> MYNLHREKIFMSYNQNKQYLEDNPEIQEKIELYGLNLLNEVISDNEEEIRADYNEANFLHPFWMNYPPLDRGKMPKGDQIPWIEVGEKAVGSKLTRLVSQREDITVREIGLPTGPDERYLLTSPTIYSLTNGFTDSIMMFVDIKS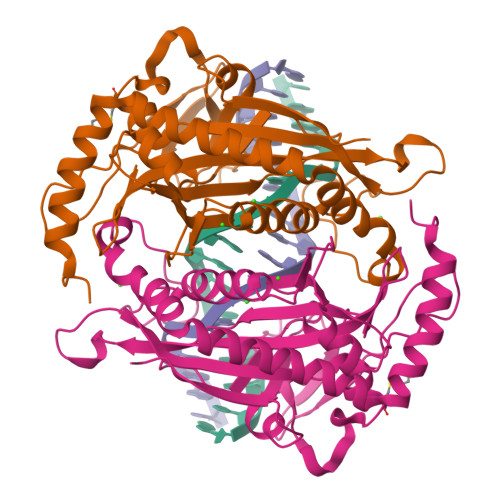VGPRDSDYDLVLSPNQVSGNGDWAQLEGGIQNNQQTIQGPRSSQIFLPTIPPLYILSDGTIAPVVHLFIKPIYAMRSLTKGDTGQSLYKIKLASVPNGLGLFCNPGYAFDSAYKFLFRPGKDDRTKSLLQKRVRVDLRVLDKIGPRVMTIDMDK>GKITLYEDRGFQGRHYECSSDHTNLQPYLSRCNSARVDSGCWMLYEQPNYSGLQYFLRRGDYADHQQWMGLSDSVRSCRLIPHSGSHRIRLYEREDYRGQMIEFTEDCSCLQDRFRFNEIHSLNVLEGSWVLYELSNYRGRQYLLMPGDYRRYQDWGATNARVGSLR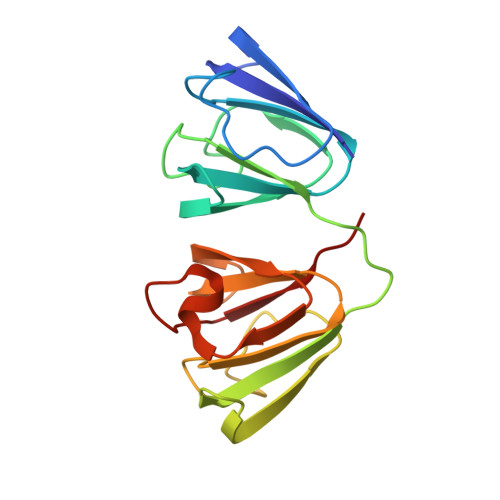RVID[2x]>[2x]GPGYQMDIPKFKRLPRHIAIIPDGNRRWALARGLEKHEGYSSGIIPGLEVYDICVKIGIGEVTFFGFTQDNTKRPQIQRKAFTDACIKSVQEIAKRDAEILVVGNTNSDIFPEELLEYTKRTKVGKGKIKINFLINYGWYWDLTYAYDNSPDGKKMIENIASAEIPRVDLLIRWGGRCRLSGMLPVQTVYSDIYVVDEMWPDFKPEHLFKALEFYQNQDITLGG

MM_0014 from the methanogenic archaeon Methanosarcina mazei is known as a versatile cis-prenyltransferase that accepts both isopentenyl pyrophosphate and dimethylallyl pyrophosphate as acceptor substrates. Cis-prenyltransferase (cPT) generally catalyzes the consecutive head-to-tail condensation of isoprene units and produces (Z,E-mixed)-polyprenyl pyrophosphates. MA1831 and MM_0014, which are orthologous cPTs from the methanogenic archaea Methanosarcina acetivorans and Methanosarcina mazei, respectively, unusually accept both IPP and DMAPP as prenyl acceptor substrates. The overall structure of MM_0014 is in a ζ-fold, which is similar to those of so far reported cPTs.

The crystals of substrate-free MM_0014 were soaked with either IPP or DMAPP to obtain its substrate-complex structures. When soaked with IPP overnight, an electron density consistent with an IPP molecule was observed in subunit A, but not in subunit B where fatty acid was still bound. IPP was bound to the cavity opening of subunit A, which remained in an open conformation and bound an inorganic phosphate molecule. Superposition of the two subunits of the IPP-binding structure (designated as “free+IPP”) showed that a fatty acid ligand overlapped IPP and therefore might inhibit the binding of the substrate to subunit B. It is also curious that no electron density derived from a Mg2+ ion was observed even though the crystallization buffer contained Mg2+. Superposition of the structures showed that the C4 of IPP, which is the atom involved in the C-C bond formation in the head-to-tail condensation, nearly overlaps the C2 of DMAPP. In fact, the position of IPP seems unsuitable for the reaction. Because of the absence of a Mg2+ ion, the pyrophosphate group of IPP is misaligned by ∼3 Å from that of DMAPP. If an allylic substrate binds to the donor-binding site, IPP is considered to move deeper into the cavity because its pyrophosphate group would be coordinated to Mg2+ along with the allylic substrate.> MSDH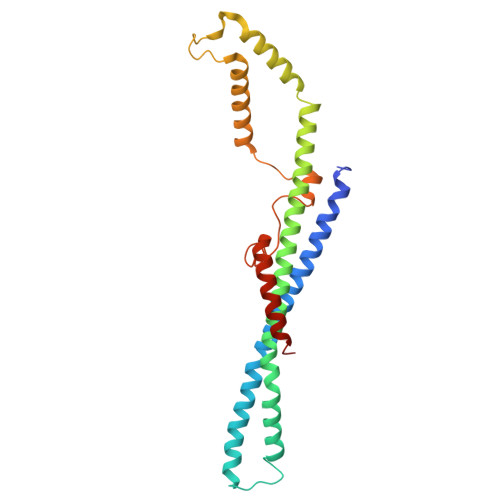TIPEYLQPALAQLEKARAAHLENARLMDETVTAIERAEQEKNALAQADGNDADDWRTAFRAAGGVLSDELKQRHIERVARRELVQEYDNLAVVLNFERERLKGACDSTATAYRKAHHHLLSLYAEHELEHALNETCEALVRAMHLSILVQENPLANTTGHQGYVAPEKAVMQQVKSSLEQKIKQMQISLTGEPVLRLTGLSAATLPHMDYEVAGTPAQRKVWQDKIDQQGAELKARGLLS> MDDCRFETSELQASVMISTPLFTDSWSSCNTANCNGSIKIHDIAGITYVAIPAVSMIQLGNLVGLPVTGDVLFPGLSSDEPLPMVDAAILKLFLQLKIKEGLELELLGKKLVVITGHSTGGALAAFTALWLLSQSSPPSFRVFCITFGSPLLGNQSLSTSISRSRLAHNFCHVVSIHDLVPRSSNEQFWPFGTYLFCSDKGGVCLDNAGSVRLMFNILNTTATQNTEEHQRYGHYVFTLSHMFLKSRSFLGGSIPDNSYQAGVALAVEALGFSNDDTSGVLVKECIET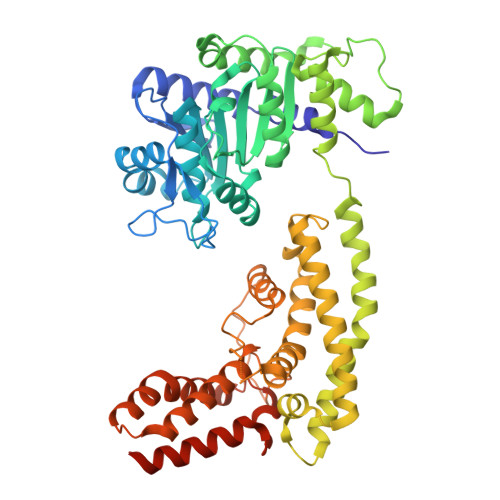ATRIVRAPILRSAELANELASVLPARLEIQWYKDRCDASEEQLGYYDFFKRYSLKRDFKVNMSRIRLAKFWDTVIKMVETNELPFDFHLGKKWIYASQFYQLLAEPLDIANFYKNRDIKTGGHYLEGNRPKRYEVIDKWQKGVKVPEECVRSRYASTTQDTCFWAKLEQAKEWLDEARKESSDPQRRSLLREKIVPFESYANTLVTKKEVSLDVKAKNSSYSVWEANLKEFKCKMGYENEIEMVVDESDAMET>MDHLPIFCQLRDRDCLIVGGGDVAERKARLLLEAGARLTVNALTFIPQFTVWANEGMLTLVEGPFDETLLDSCWLAIAATDDDTVNQRVSDAAESRRIFCNVVDAPKAASFIMPSIIDRSPLMVAVSAGGTSPVLARLLREKLESLLPQHLGQVARYAGQLRARVKKQFATMGERRRFWEKFFVNDRLAQSLANADEKAVNATTERLFSEPLDHRGEVVLVGAGPGDAGLLTLKGLQQIQQADIVVYDRLVSDDIMNLVRRDADRVFVGKRAGYHCVPQEEINQILLREAQKGKRVVRLKGGDPFIFGRGGEELETLCHAGIPFSVVPGITAASGCSAYSGIPLTHRDYAQSVRLVTGHLKTGGELDWENLAAEKQTLVFYMGLNQAATIQEKLIAFGMQADMPVALVENGTSVKQRVVHGVLTQLGELAQQVESPALIIVGRVVALRDKLNWFSNH[2x]

Siroheme is the modified isobacteriochlorin tetrapyrrole used by siroheme-dependent sulfite and nitrite reductases (SiR/NiRs) in catalyzing the six-electron reduction of sulfite to sulfide or nitrite to ammonia. CysG is encoded by a gene fusion between a C-terminal SUMT (CysGA) and an N-terminal bifunctional dehydrogenase/ferrochelatase (CysGB). The N-terminal enzyme module, CysGB, is a three-domain bifunctional dehydrogenase/ATP-independent class III ferrochelatase12 that performs the final two steps of siroheme biosynthesis. The C-terminal enzyme module, CysGA, is homologous to a well-studied class of SAM-dependent uro’gen III methyltransferases (SUMTs) that catalyzes the methylations to generate precorrin-210,13.

A soak experiment with precorrin-2 and NADH resulted in a structure with low-occupancy precorrin-2 bound to one active site but NADH, also at low occupancy, bound to the other. Precorrin-2 is less oxidatively stable than more highly conjugated tetrapyrroles, and this was apparent in the weaker density of the central ring and partial occupancy of the molecule as a whole. Precorrin-2 is a highly oxygen-sensitive dipyrrocorphin that lacks the ring conjugation of the later, more stable, isobacteriochlorins, sirohydrochlorin and siroheme. Nevertheless, we see similar changes to the conformation of the helical domain and surrounding loops that are associated with tetrapyrrole binding, so we were able to assign a binding position for precorrin-2 that positions C15 towards the Rossmann fold. Interestingly, in the precorrin-2 bound structure, D104 is in two conformations whose occupancies correspond to the partial occupancy of the precorrin-2 molecule. Consequently, although both tetrapyrroles coordinate positively charged amino-acid side chains with their eight carboxylates, the ring of the less rigid precorrin-2 is not as ordered as it is in the sirohydrochlorin. Precorrin-2, oriented with the C2 and C7 methyl groups buried in hydrophobic pockets and coordinated by positively charged amino acids at each corner, presents C15 toward the Rossmann fold where a tightly docked NAD+ places its nicotinamide ring.> MSSQSSNTESLSRFPLWQVITPVRRKVILAMALAGLAALTSLGALLFLAWSLRDIRATPDAIPAWPLGGVIGCVVLTFVLRLQAFNTSHYAAFHLENILRSRLARKALQLPPGVLQQMGSGSVAKVMLDDVKSLHIFVADSTPLYARAIIMPLATIVILFWLDWRLAIATLGVLAFGSVVLVLARQRSENMAQRYHKAREQVSAAVIEFVQAMPVVRTFDSGSTSFLRYQRALEEWVDVLKTWYRKAGFSARFSFSILNPLPTLFVLIWSGYGLLHYGSFDFIAWVAVLLLGSGMAEAVMPMMMLNNLVAQTRLSIQRIYQVLAMPELSLPQSDQQPQEASITFEQVSFHYPQARTGAALQEVSFHVPAGQIVALVGPSGAGKSTVARLLLRYADPDKGHIRIGGVDLRDMQTDTLMKQLSFVFQDNFLFADTIANNIRLGAPDTPLEAVIAAARVAQAHDFISALPEGYNTRVGERGVFLSGGQRQRITIARALLQDRPILVLDEATAFADPENEAALIKALAAAMRGRTVIMVAHRLSMVTQADVILLFSDGQLRE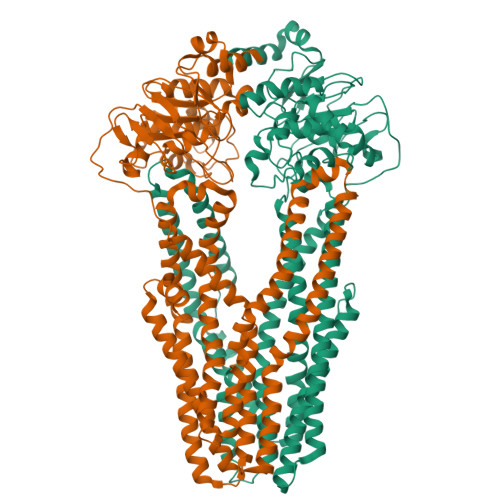MGNHTQLLAQGGLYQRLWQHYQQAQHWVPGGTQEEVVENERQ;> MKDNNPADNLAWRVIWRQLISSVGSQARMLRRSMLALLLAAFMQGIAFACLYPIIDALLRGDAPQLLNWAMAFSVAAIVTLVLRWYGLGFEYRGHLAQATHELRLRLGEQLRRVPLEKLQRGRAGEMNALLLGSVDENLNYVIAIANILLLTIVTPLTASLATLWIDWRLGLVMLLIFPLLVPFYYWRRPAMRRQMQTLGEAHQRLSGDIVEFAQGMMVLRTCGSDADKSRALLAHFNALENLQTRTHRQGAGATMLIASVVELGLQVVVLSGIVWVVTGTLNLAFLIAAVAMIMRFAEPMAMFISYTSVVELIASALQRIEQFMAIAPLPVAEQSEMPERYDIRFDNVSYRYEEGDGHALNHVSLTFPAASMSALVGASGAGKTTVTKLLMRYADPQQGQISIGGVDIRRLTPEQLNSLISVVFQDVWLFDDTLLANIRIARPQATRQEVEEAARAAQCLEFISRLPQGWLTPMGEMGGQLSGGERQRISIARALLKNAPVVILDEPTAALDIESELAVQKAIDNLVHNRTVIIIAHRLSTIAGAGNILVMEEGQVVEQGTHAQLLSHHGRYQALWQAQMAARVWRDDGGSASGEWVHE>MSKSVFVGELTWKEYEARVAAGDCVLMLPVGALEQHGHHMCMNVDVLLPTAVCKRVAERIGALVMPGLQYGYKSQQKSGGGNHFPGTTSLDGATLTGTVQDIIRELARHGARRLVLMNGHYENSMFIVEGIDLALRELRYAGIQDFKVVVLSYADFVKDPAVIQQLYPEGFLGWDIEHGGVFETSLMLALYPDLVDLDRVVDHPPATFPPYDVFP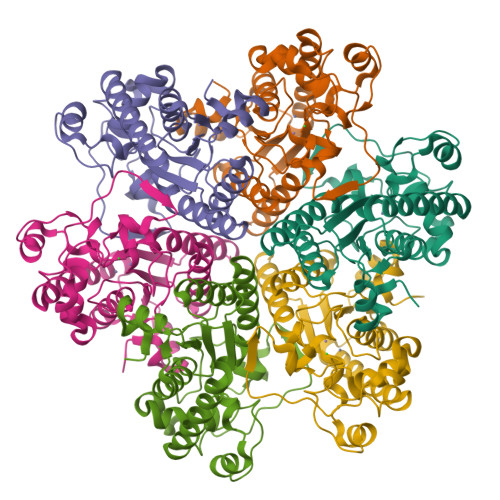VDPARTPAPGTLSSAKTASREKGELILEVCVQGIADAIREEFPPT[6x]> EPTLVPTPPPELPTDCGGPFELWEPNTTFSSTNFPNSYPNLAFCVWILNAQKGKNIQLHFQEFDLENINDVVEIRDGEEADSLLLAVYTGPGPVKDVFSTTNRMTVLLITADVLARGGFKANFTTGYHLGIPEPCKADHFQCKNGECVPLVNLCDGHLHCEDGSDEADCVRFFNGTTNNNGLVRFRIQSIWHTACAENWTTQISNDVCQLLGLGSGNS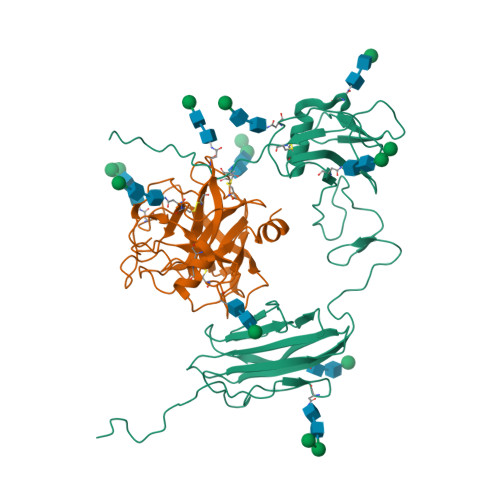SKPIFPTDGGPFVKLNTAPDGHLILTPSQQCLQDSLIRLQCNHKSCGKKLAAQDITPK;> IVGGSNAKEGAWPWVVGLYYGGRLLCGASLVSSDWLVSAAACVYGRNLEPSKWTAILGLHMKSNLTSPQTVPRLIDEIVINPHYNRRRKDNAIAMMHLEFKVNYTDYIQPICLPEENQVFPPGRNCSIAGWGTVVYQGTTANILQEADVPLLSNERCQQQMPEYNITENMICAGYEEGGIDSCQGDAGGPLMCQENNRWFLAGVTSFGYKCALPNRPGVYARVSRFTEWIQSFLH>GSHMASSHLAELVASAKAAISQASDVAALDNVRVEYLGKKGHLTLQMTTLRELPPEERPAAGAVINEAKEQVQQALNARKAELESAALNARLAAETIDVSLPGRRIENGGLHPVTRTIDRIESFFGELGFTVATGPEIEDDYHNFDALNIPGHHPARADHDTFWFDTTRLLRTQTSGVQIRTMKAQQPPIRIIAPGRVYRNDYDQTHTPMFHQMEGLIVDTNISFTNLKGTLHDFLRNFFEEDLQIRFRPSYFPFTEPSAEVDVMGKNGKWLEVLGCGMVHPNVLRNVGIDPEVYSGFAFGMGMERLTMLRYGVTDLRSFFENDLRFLKQFK[2x];>[2x]MKFSELWLREWVNPAIDSDALANQITMAGLEVDGVEPVAGSFHGVVVGEVVECAQHPNADKLRVTKVNVGGDRLLDIVCGAPNCRQGLRVAVATIGAVLPGDFKIKAAKLRGEPSEGMLCSFSELGISDDHSGIIELPADAPIGTDIREYLKLDDNTIEISVTPNRADCLGIIGVARDVAVLNQLPLVQPEIVPVGATIDDTLPITVEAPEACPRYLGRVVKGINVKAPTPLWMKEKLRRCGIRSIDAVVDVTNYVLLELGQPMHAFDKDRIEGGIVVRMAKEGETLVLLDGTEAKLNADTLVIADHNKALAMGGIFGGEHSGVNDETQNVLLECAFFSPLSITGRARRHGLHTDASHRYERGVDPALQHKAMERATRLLIDICGGEAGPVIDITNEATLPKRATITLRRSKLDRLIGHHIADEQVTDILRRLGCEVTEGKDEWQAVAPSWRFDMEIEEDLVEEVARVYGYNNIPDEPVQASLIMGTHREADLSLKRVKTLLNDKGYQEVITYSFVDPKVQQMIHPGVEALLLPSPISVEMSAMRLSLWTGLLATVVYNQNRQQNRVRIFESGLRFVPDTQAPLGIRQDLMLAGVICGNRYEEHWNLAKETVDFYDLKGDLESVLDLTGKLNEVEFRAEANPALHPGQSAAIYLKGERIGFVGVVHPELERKLDLNGRTLVFELEWNKLADRVVPQAREISRFPANRRDIAVVVAENVPAADILSECKKVGVNQVVGVNLFDVYRGKGVAEGYKSLAISLILQDTSRTLEEEEIAATVAK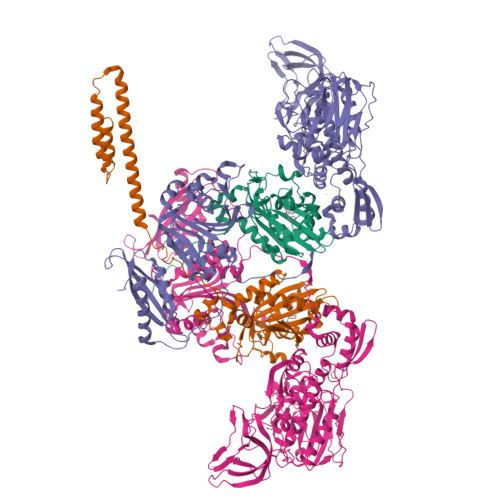CVEALKERFQASLRD> SNAMMELPGQPSLTDGGAALFAWLRTMRNEHPVWRDQFGIYHVFRYDDVRQILGDYQTFSSDRTRLMPTAQGFGKGGITMIDPPEHRHQRRLITHAFTPQSISAMEPRIRQIADHLLDELPGPEFDLVEHFAYPLPVIVIAELLGVPPGDRHLFRTWSDRLMSLQVENYADPELARTVAAAMTEMNDYLREHCRSRRTHPRDDLLTRLVQAEVEGKRLDLEEVVNTASLLLLAGHLTTTVLIGNTMLCLWDHPEAEKAVRADPSLIPAALEESLRLRSPFLQA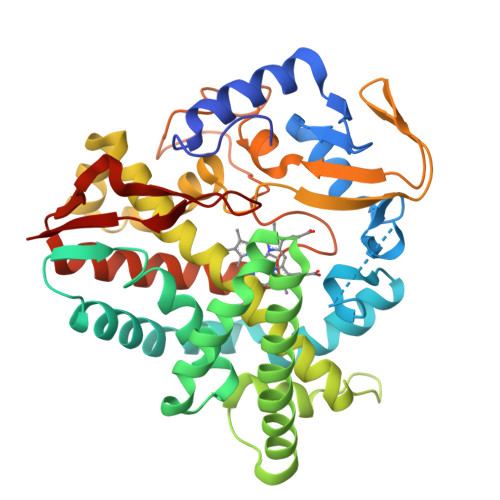GRVTTRDVTIAGETIPANRFVMAWILSANHDDRRFPDPERFDLHRQTTGHIAFGHGVHFCLGAQLGRLEGRIALERLLGRFTEIHPWPREGISFYQSAIFGASRMPVRCG> MIHCLRNIRTVSALQSKISYNLGGGNKRKKTSGDLDNYDVLFVGANLGGICSNHFDKDTHGKYKCFVSFDQPINQIYSVRIPYEQQRVRKSEYIHFSKKSINQFTPSEMLAVKEILPEQNAVVLSSGRRIGYNQLVLATGLKHDFSQIKGFYEALEHPEHPVYANRDPETWRSAQHKYSKYISNFKSGDGYFCIPEYPYAGEVECFNFFVSDEVWKWAQH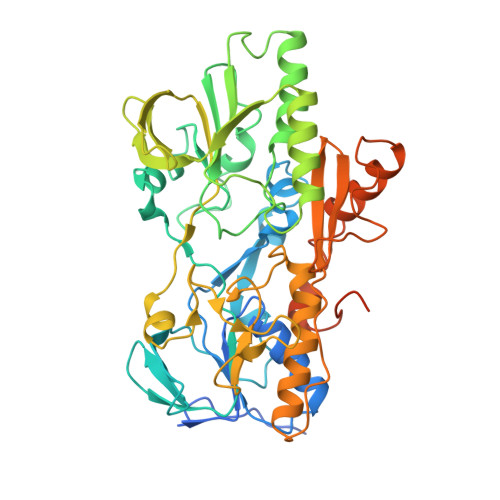HGALSPKHTFTIVNANEKFVHYCDSADAFIKERLEKRGIRVEYNTKLLEVHQDGQKATFINTKTGEKSVRDYNNLYSIVPSKRQEFLDKAGLTNGNGLLNVDHQTLQHKKYKNIFGLGDAADLPTTKTFWAGWYQIAVVRNNVKRNLQGQTLNAHYDGFSKVPLFTGHQTLTYVAHSYGGVGNWQHLKHNNGGILAWMRYRSWAKGMAKKFQDFYNGARLGPPYHKVLKSFPELPGSPESQQSSGISKYFPTKTENKAAH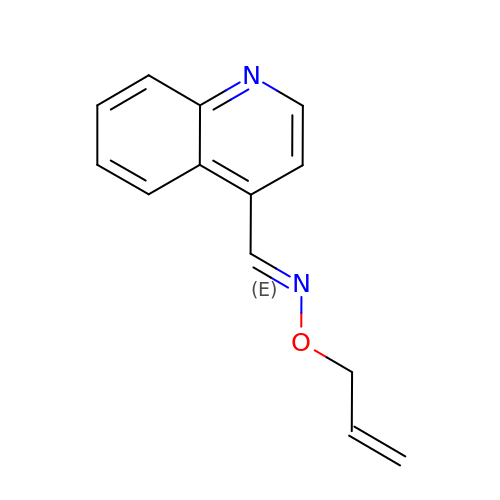(E)-N-(prop-2-en-1-yloxy)-1-(quinolin-4-yl)methanimine | C13 H12 N2 O | QNCJWFLSMPZQBD-XNTDXEJSSA-N>GSHMNGSIQGKPLLGKGMSESLTGTLDAPFPEYQTLPADPMSVLHNWLERARRVGIREPRALALATADSQGRPSTRIVVISEISDAGVVFSTHAGSQKGRELLHNPWASGVLYWRETSQQIILNGQAVRLPNAKADDAWLKRPYATHPMSSVSRQSEEL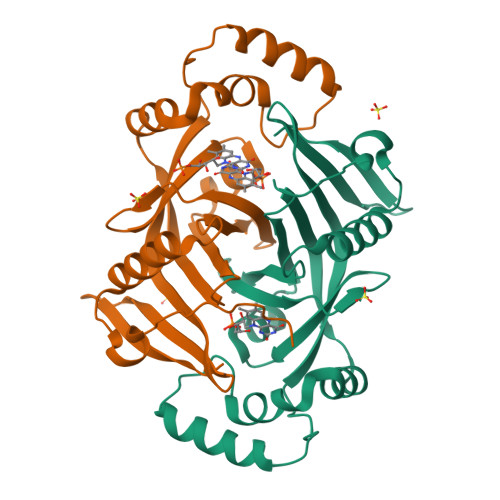QDVQAMRNAARQLAELQGPLPRPEGYCVFELRLESLEFWGNGQERLHERLRYDRSDTGWNVRRLQP[2x]>[3x]AS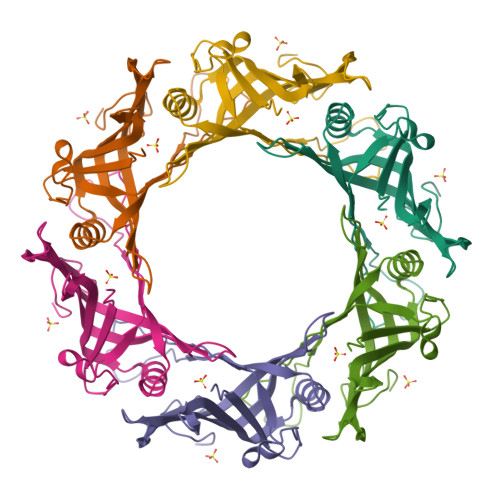MKDIYVEFRGKYKVDGESRDSEHKGWLEVNSWSHNIRQPKSATSSSVGGHTAERVEHSDMVFVKDLDATSPKLWEACSAGYTFDEVQIDFYRANGDKRIKYLQIKLKHVLVSSVTPTVNEEGVPTEAFGLKYAAVEWTYNQQDINGTAKGAVTKKWSLSNNTASYAALA GM1-Gangliosidosis and Morquio B disease are two manifestations of mutations on the GLB1 gene that encodes the vital lysosomal β-galactosidase. This enzyme is responsible for removal of a β-galactosyl residue from the non-reducing end of its substrate, converting gangliosides GM1 and GA1 into GM2 and GA2, respectively. Based on X-ray crystallographic studies of compounds 1, 14, 16, 17 as well as 22 and 31 in complex with Cellvibrio japonicus β-galactosidase (CjGH35), a tractable bacterial model which shows around 27% sequence identity with the human enzyme, notably conserved active centers, intensities of inhibition and chaperoning properties, may be partially rationalized. For the inhibitors studied here, the ligand sugar moieties have clear density in all the active sites and overlay with ring C atoms 2 to 5 in similar positions.

Ligand 31 is identical to 17 apart from lacking a hydroxyl group at C-2, the importance of which is reflected in a much poorer Ki value (200-fold worse for human lysosomal β-galactosidase). The active site residues are similarly oriented in all of the structures, with slight differences for 31. There are two other differences in the ligand interactions of 31 (not only from those seen for 17, but also from the other complexes studied here). Firstly, there is a hydrogen bond from the C-3 hydroxyl to ND2 Asn204, in addition to the three hydrogen bonds to Asn67, Lys134 and a water molecule (which is hydrogen bonded to OD1 Asn204 and OE1 Gln64). Secondly, there is a shift in the position of Gln64, with the NE2 atom forming a hydrogen bond to O Ala348, instead of the OE1 interacting with a water which is hydrogen bonded between O Thr65 and ND2 Asn67 (as seen in the other structures). These probably play a far lesser contribution to the weaker Ki values than the absence of three potential hydrogen bonds from a C-2-OH group. The importance of this interaction is clearly seen in comparing the Ki value of the GH35 bovine β-galactosidase with 17 and 31. These inhibitors differ only in the presence of the hydroxyl group at that position, and indeed 31 binds some 20 fold less tightly, corresponding to an approximate 2 kcal/mol difference. An even bigger 200 fold affinity difference is seen for the human lysosomal β-galactosidase (GH35), implying crucial interactions of this particular hydroxyl group with GH35 enzymes. The corresponding deoxy derivative 31 exhibited distinctly reduced chaperoning activity and was only trailed by deoxyfluoro analog 37. For the cyclopentanoid chaperones, on the other hand, OH-2 appears to be a vital feature for their activity as inhibitors and pharmacological chaperones, since its absence and the concomitantly increased basicity of the adjacent amine apparently cannot compensate for the reduced number of interactions with amino acid residues resulting from the removal of this particularly crucial functional group.

>MGSSHHHHHHAAPLPELLSNNGKHALMVDGAPYIILGSQTNNSSNYPDALKDVWPSMEKMGANTLSIPVAWEQIEPVEGQFDFSFVDVLLKEARQRKVRLVLLWFATWKNNAPHYAPAWVKLDNARFPRVVKEDGDTLNSLSPLGQNTLAADKKAFVELMKYLAKRDKDHTVIMVQVQNEVGTYGAVRDYSPMAQAVFNAAVPDDLIQKLQLKPGTWSQVFGRDADEFFHAYQIARYCDEVTVAGKAIKNLPMYVNVALRNPFNPGLPGQYSSGGGTDNVLHIWKAAAPNIDLIAPDIYFRDYKTVSKVLELYTRPDNALFVAEIGNDQPFARYLFPTLGKGGIGFSPFGMDDTDYTNYPLGAKVYNDETIEQFAQVYRLVNPMMREWARLSYQGQVWGVAEPLDSTTETQKIWNAEATPEEKEQHKKDRASALTQQLDLGLWDAEVTYGRPMFWVTPPEGNTPAAGGALIAQLDDNEYLVTAYKARVEFKPSQELAGKKFMIERVEEGRFEKGKWVMERVWNGDQTDWGLNFTDRPHLLRVKMASYSVQ[8x]>[2x]MHKLLLALLSLSLVGCIDSKEEILEEKNQGLVYCAEANPVSFNPQVTTTGSTIDIIANQLYDRLISIDPVTAEFKSELATDWKISKDGKSVTFTLRKGVKFHTTAYFTPTREFNADDVIFTFSRLFDVYNPYHFVGDANYPYFQSVGIDQLIRKIVRVSDHQVRFELFNAESSFLANMATDFAVVLSKEYAMALKANNQENLFDQYPVGTGPYIYKEYRRDHLVRFYKNADYWKHEVALEQLVYDITPNGTTRIAKILTKECDVTAHPSSAQLSILAQRDDINVERETNLNIGYWAFNTERPPFDNLKVRQALVHAIDIEKIMQAVYYGNGLRARSILPPTSWAFEPQKNMPIFDPQLAKKLLTEAGYEKGFDMSIWAMPVSRIYNPNARKMAELMQSDLRKIGVNVNIVEYEWNTFIQRIGEHRHDSVLLGWAADTPDPDNFF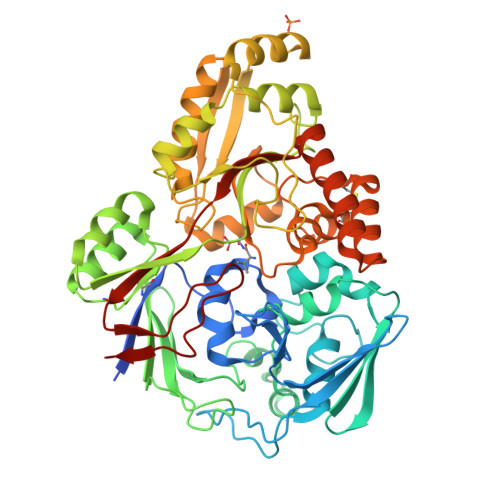SPLLSCTATFSGKNPANWCNPEFDLLLTKALDTTDLNLRKQYYDAAQSMIIEQLPLYPIAHGMRFQASSADVEGITLGPFGAISLANARKKHHHHHH5-aminocarbonyl-3-nitrophenyl 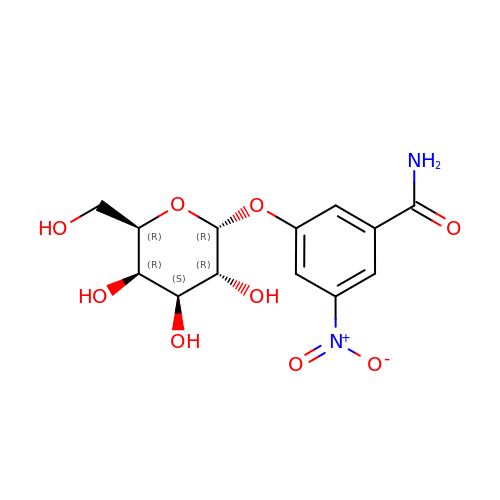alpha-D-galactopyranoside | C13 H16 N2 O9 | BYSXBFJVGIOFBO-LNSPPBFMSA-N> DDRDLLLAPKWISFLSLSSFLKQKLLSLLRQIRELRLTTTVYPPQDKLMWWSHCCDPEDIKVVILGQDPYHKGQATGLAFSVDPQCQVPPSLRSIFRELEASVPNFSTPSHGCLDSWARQGVLLLNTVLTVEKGRAGSHEGLGWDWFTSFIISSISSKLEHCVFLLWGRKAIDRTPLINAQKHLVLTAQHPSPLASLGGRHSRWPRFQGCNHFNLANDYLTRHRRETVDWGLLEQ

Efficient γ-herpesvirus lytic phase replication requires a virally encoded UNG-type uracil-DNA glycosylase as a structural element of the viral replisome. Uniquely, γ-herpesvirus UNGs carry a seven or eight residue insertion of variable sequence in the otherwise highly conserved minor-groove DNA binding loop. The UNG leucine loop is a conserved structural feature which is responsible for widening the DNA minor groove and flipping pyrimidines out of the base stack and, in the case of uracil, into the UNG active site for catalysis. kUNG, in common with other known UNGs, comprises a single C-terminal globular domain made up of a four-stranded parallel β-sheet flanked by six α-helices, with an additional left-handed coil of three helices at the N-terminus.

The structure of kUNG in its apo form was solved in two different crystal forms. The disc-shaped structure of the leucine loop extension centred on the side chain of Q212 was not observed in the two unbound kUNG structures. Taken together, the unbound kUNG structures suggest that the leucine loop extension is highly flexible in solution. However, the absence of electron density for the leucine loop insertion in the apo kUNG C2 crystal form, and partial ordering of the leucine loop along with significant crystal contacts in the P21 crystal form indicate that the leucine loop is very likely highly mobile in solution. Mutagenesis suggests a model in which the kUNG loop is pinned outside the DNA-binding cleft until DNA docking promotes rigid structuring of the loop and duplex nucleotide flipping, a novel observation for UNGs.> VIPEGYTQENVAVRGKATQSAQLRGEHAANSEASNAIDGNRDSNFYHGSCTHSSGQANPWWRVDLLQVYTITSVTITNRGDCCGERISGAEINIGQHLASNGVNNPECSVIGSMATGETKTFHCPAPMIGRYVVTYLPTSESLHLCEVEVNVDK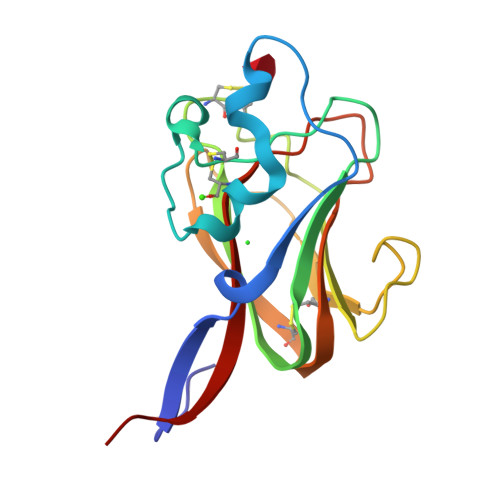PAAA>[6x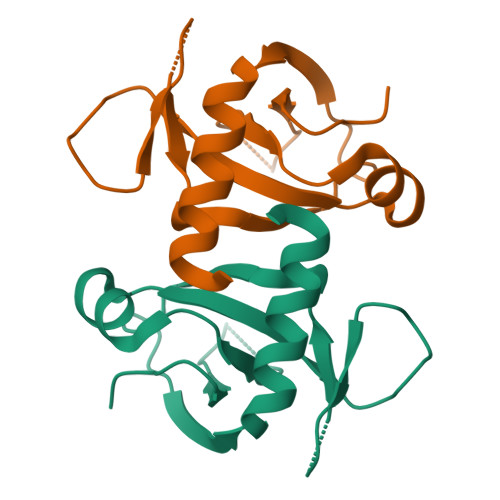]MVSRYVPDMGDLIWVDFDPTKGSEQAGHRPAVVLSPFMYNNKTGMCLCVPCTTQSKGYPFEVVLSGQERDGVALADQVKSIAWRARGATKKGTVAPEELQLIKAKINVLIG(4-AMINO-2-METHYLPYRIMIDIN-5-YL)METHYL DIHYDROGEN PHOSPHATE | 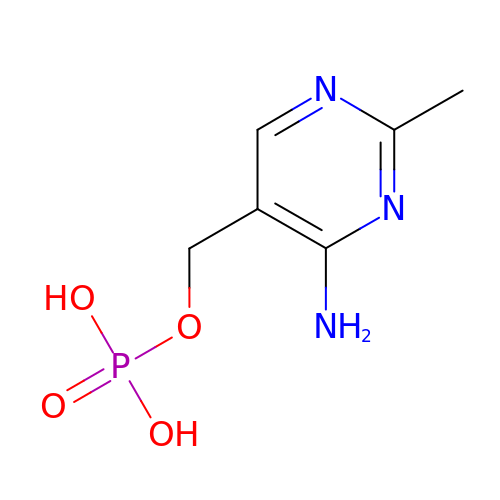C6 H10 N3 O4 P | PKYFHKIYHBRTPI-UHFFFAOYSA-N>[2x]MGEKITEEREFQSISEIPEEEIDATNDEEKLADIVENEIEKEIRKSKTRKCKTIENFYYYILRDGKIYPASDYDIEVEKGKRS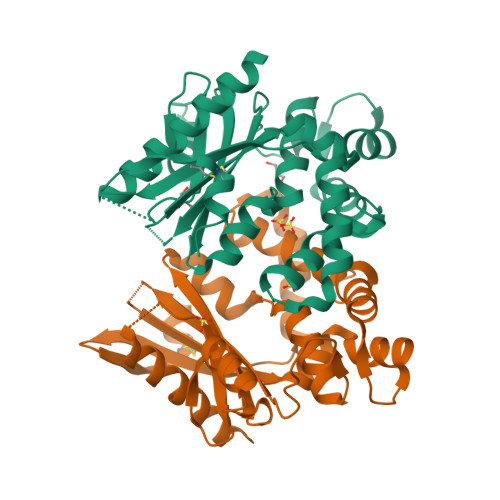ANDIYAFVETDVTRDFDEFLFDIDYGLPSISDILKFYLEKAGFRIANEVPTPNLKYYIHAVVEFGEDRPQYLAVNIYDIDSLARALRIPQIVEQKLGNKPRTITADEFNDIERIVAEEQPILAGYTYDEALRIPYHYYVDHNNSFKDDALKIAHAYLQLFPTPYQVCYEWKARWFNKIDCLKLERLKPSSHHHHHH>MGSSHHHHHHSGLVPRGSHMAGARTQELVQQRTQGLLEKVINERLVALARAQVSQIQRELEYPLTVVHGLANSTRLLGEPGADGMPQLNASRDEISALLRSTVQNNPKLLDTFMAWEPNAFDTDAAFAGQPGKGYGPDGRYLPWWYRGADGKPIVEAMADSIDSEKLLPTGVRENEFYACPKENKRPCIIDPAPYEMGGKTVMMSSFNVPIMVGDQFRGAVGADLSLAFIQDLLKRADQQLYDGAGEMALIASNGRLVAYTRDDSKLGEPAGSVLDGNEVDNLKNLTVDQPLYDIDAEHGHIELFLPFTIADSGVRWTLMLQIPQAAVFGELQQLQGELSDQRQQDILGM[2x]

Chemoeffectors are sensed by chemoreceptors that in turn stimulate chemosensory pathways that modulate the activity of the flagellar motor. A canonical chemoreceptor is composed of an extracytosolic ligand-binding domain (LBD) and a cytosolic region that contains the signaling domain that interacts with other signaling proteins. The dCache domain is the predominant extracellular LBD in bacterial signal transduction systems, and it is present in about 15% of all chemoreceptors. To identify the molecular determinants for acetylcholine recognition, we report high-resolution structures of PctD-LBD (with bound acetylcholine and choline) and PacA-LBD (with bound betaine).

We demonstrate that this chemoattraction is mediated by the PctD (PA4633) chemoreceptor. Acetylcholine and choline bound with high affinity, with dissociation constants of 23 and 2.6 μM, respectively. Crystals formed in the presence of acetylcholine and choline, and atomic structures were determined and refined to a resolution of 1.8 and 2.0 Å, respectively. The structures showed the typical dCache fold, and alignments with all structures present in the protein data bank showed that it is most similar to the LBD of the TlpQ chemoreceptor from P. aeruginosa in complex with histamine, another neurotransmitter. Well-defined electron density was observed for choline and acetylcholine, which permitted the precise placement of ligand structures. As in the majority of dCache domains, the ligand was bound to the membrane-distal module. The quaternary amine moiety of both ligands is coordinated by hydrophobic interactions with a number of aromatic amino acids (Phe124, Phe188, Tyr206, and Trp155) and two methionine residues (Met169 and Met215). However, the tails of the two ligands point in opposing directions. The choline tail interacts with Ser217 and Asp235, whereas the acetylcholine tail interacts with Ala168, Asp171, and Ser172.> SSLPMARYYIIKYADQKALYTRDGQLLVGDPVADNCCAEKICTLPNRGLDRTKVPIFLGIQGGSRCLACVETEEGPSLQLEDVNIEELYKGGEEATRFTFFQSSSGSAFRLEAAAWPGWFLCGPAEPQQPVQLTK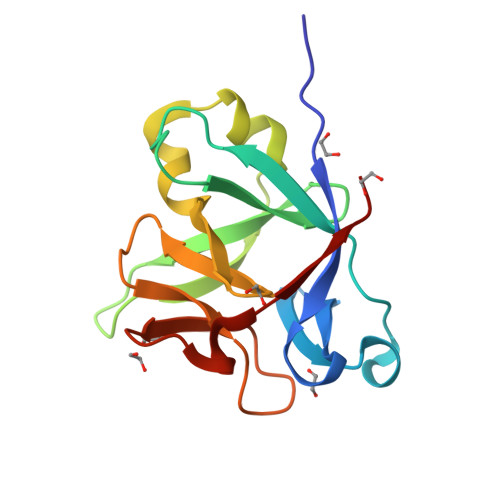ESEPSARTKFYFEQSW4-propylbenzenesulfonamide 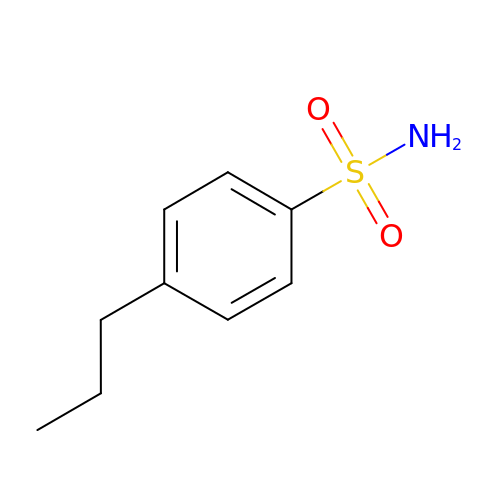| C9 H13 N O2 S | CICCMHNIYTXWRF-UHFFFAOYSA-N>[2x]SHHHHHHGSELPQMVQQLN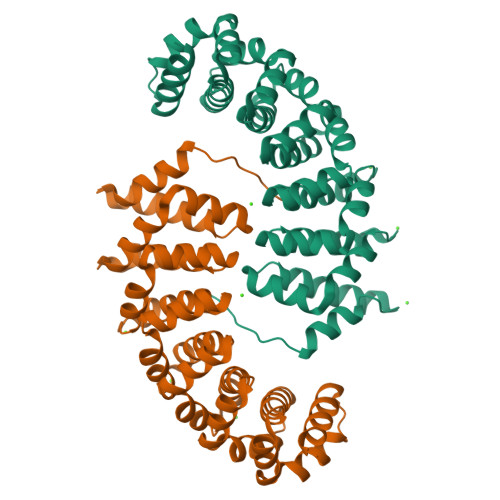SPDQQELQSALRKLSQIASGGNEQIQAVIDAGALPALVQLLSSPNEQILQEALWTLGNIASGGNEQIQAVIDAGALPALVQLLSSPNEQILQEALWTLGNIASGGNEQIQAVIDAGALPALVQLLSSPNEQILQEALWTLGNIASGGNEQIQAVIDAGALPALVQLLSSPNEQILQEALWTLGNIASGGNEQIQAVIDAGALPALVQLLSSPNEQILQEALWTLGNIASGGNEQKQAVKEAGAEPALEQLQSSPNEKIQKEAQEALEKIQ>MTETTENVVITIPDKTSFTFHEAATSPSEGEEFVVGHFRELTVKISGSSTSREIKFYAVDENGEKTALSGTNKTDFQLGSS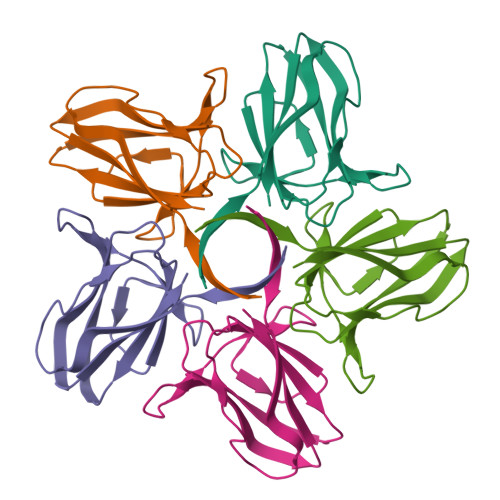TLNTNEYWDFDIAGLFKVMFEVVSVTGDVTVKGIVVS[5x]>[4x]MWAFPERFEGRHVRLEPLALAHLPAFLRHYDPE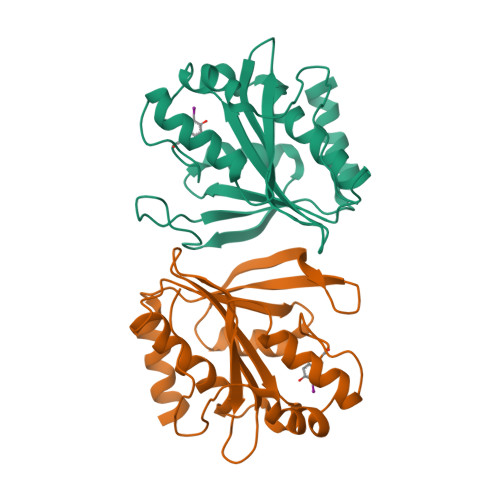VYRFLSRAPVAPTEEALRAHLEGLLGEPGRVNWAILFGKEVAGRISVIAPEPEHAKLELGTMLFKPFWGSPANKEAKYLLLRHAFEVLRAERVQFKVDLRNERSQRALEALGAVREGVLRKNRRLPDGAFRDDVVYSVLKEEWPGVKARLEARLYGASGNP>MTNNKYTNRPIHQLQELLRLNGVDEEWEPILLPALMTLEDSYLEWMAAGEGYIPPRDRLLAAFSTLRPNEVRYILFGQDPGPRPESAIGYAFIDGRVREIFSPRGLSREVNR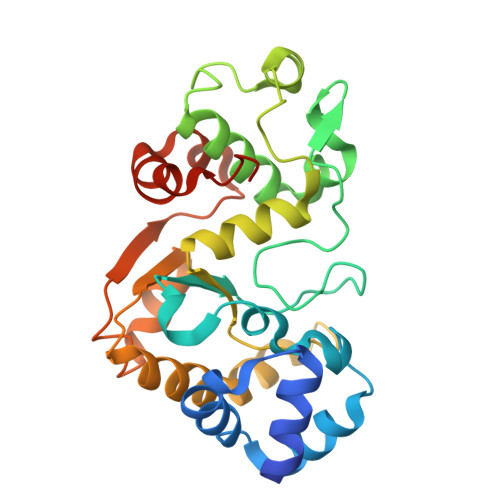ATSLRNFIKMALVARGSLDPRDTSQEAIAALDKTLLVSQMRELRENFERSGVLLLNMALLFTSKEESRRHIRAWRAFIEKLLEGFEAYGPTLILFGAHAREVQKLKSARGLPQVALEHPYNHTFIVNEKAWELFGPMDLLLKRLEHHHHHH[2x]>GSETQQVPTEEVSLEVLLSNGQKVLVNVLTSDQTEDVLEAVAAKLDLPDDLIGYFSLFLVREKEDGAFSF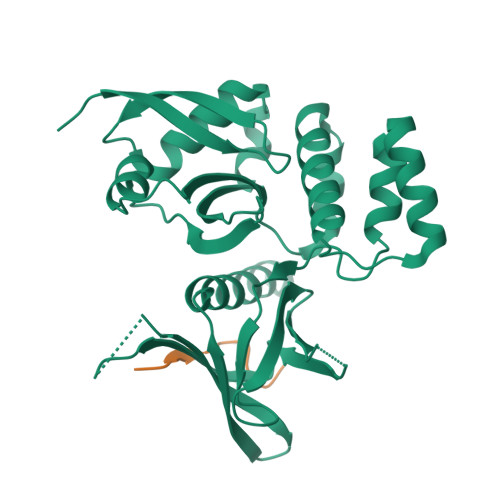VRKLQEFELPYVSVTSLRSQEYKIVLRKSYWDSAYDDDVMENRVGLNLLYAQTVSDIERGWILVTKEQHRQLKSLQEKVSKKEFLRLAQTLRHYGYLRFDACVADFPEKDCPVVVSAGNSELSLQLRLPGQQLREGSFRVTRMRCWRVTSSVPLPSGSTSSPGRGRGEVRLELAFEYLMSKDRLQWVTITSPQAIMMSICLQSMVDELMVKKSGGS[3x];>GPLGSPADTCIYNPLFGSD[3x]{2-[5-hydroxy-4-(hydroxymethyl)-6-methylpyridin-3-yl]ethyl}phosphonic acid | C9 H14 N O5 P | 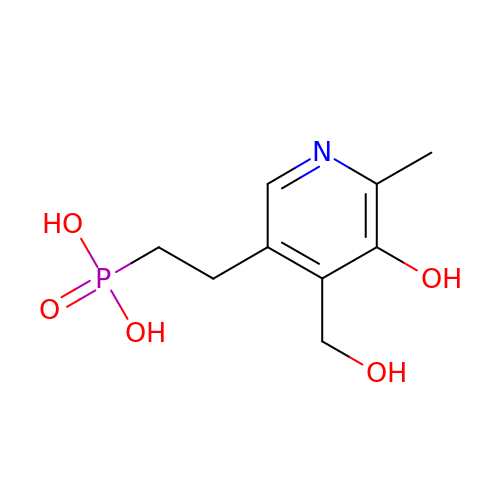JWJVWJVYBWLXDN-UHFFFAOYSA-N>[2x]STGSAMSQKHLQINQTFEELRLVTQDTENELKKLQQTQEYFIIQYQESLRIQAQFGPLAQLSPQERLSRETALQQKQVSLEAWLQREAQTLQQYRVELAEKHQKTLQLLRKQQTIILDDELIQWKRRQQLAGNGGPPEGSLDVLQSWCEKLAEIIWQNRQQIRRAEH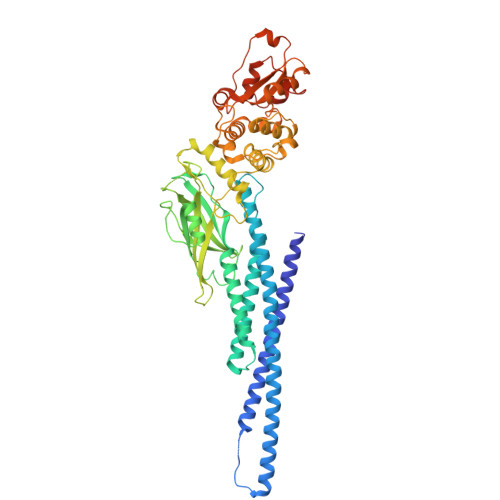LCQQLPIPGPVEEMLAEVNATITDIISALVTSTFIIEKQPPQVLKTQTKFAATVRLLVGGKLNVHMNPPQVKATIISEQQAKSLLKNENTRNDYSGEILNNCCVMEYHQATGTLSAHFRNMSLKRIKRSDRRGAESVTEEKFTILFESQFSVGGNELVFQVKTLSLPVVVIVHGSQDNNATATVLWDNAFAEPGRVPFAVPDKVLWPQLCEALNMKFKAEVQSNRGLTKENLVFLAQKLFNNSSSHLEDYSGLSVSWSQFNRENLPGRNYTFWQWFDGVMEVLKKHLKPHWNDGAILGFVNKQQAHDLLINKPDGTFLLRFSDSEIGGITIAWKFDSQERMFWHLMPFTTRDFSIRSLADRLGDLNYLIYVFPDRPKDEVYSKYYTPVPCESATAKAVDGYVKPQ> IPIFL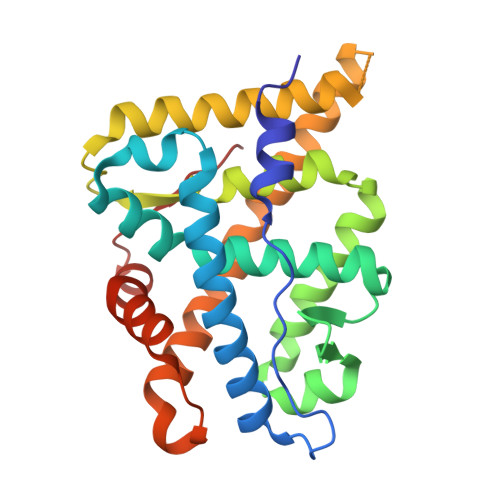SVLQSIEPEVVYAGYDNTQPDTSASLLTSLNELGERQLVRVVKWAKALPGFRNLHVDDQMTLIQYSWMGVMVFAMGWRSYKNVNSRMLYFAPDLVFNEQRMQKSTMYNLCVRMRHLSQEFVWLQVTQEEFLCMKALLLFSIIPVEGLKNQKYFDELRMNYIKELDRVISFQGKNPTSSSQRFYQLTKLLDSLQDLVRKLHQFTFDTFVQSQSLSVEFPEMMSEIISAQVPKILAGMVKPLLFHKQ Cytosolic sulfotransferases (SULTs) comprise a family of enzymes that catalyze the transfer of a sulfonate group from 3′-phosphoadenosine 5′-phosphosulfate (PAPS) to an acceptor group of the substrate. In doing so, SULTs modulate the activities of a large array of small endogenous and foreign chemicals, including drugs, toxic compounds, steroid hormones, and neurotransmitters. As expected, all SULTs share the same basic fold: a central four-stranded parallel β-sheet surrounded by α-helices and three loops that are often disordered (dashed lines) in the absence of PAP and/or substrate. The crystal structures of SULT1C3 bound to PAP, apo SULT1C2, a ternary complex of SULT1C2 bound to PAP, and the environmental toxin, pentachlorophenol (PCP), and SULT4A1 were solved at 3.2, 2.0, 1.8, and 2.2 Å, respectively.

SULT4A1 is one of the hSULTs that is most divergent in sequence, and examination of the binding pocket revealed two significant differences that are predicted to affect PAP binding. First, a Trp in α3 that is conserved in all other hSULTs and stacks with the adenine ring of PAPS (Trp53 in SULT1A1) is replaced with a Leu in SULT4A1. Second, the magenta PAP binding loop is much shorter in SULT4A1 than in the other hSULTs, and lacks the conserved Lys residue that separates the key PAPS binding residues Arg258 and Gly260 (SULT1A1 numbering), which results in these residues being out of register. Taken together, SULT4A1 has a slightly smaller PAPS binding pocket that is predicted to be unable to accommodate the cofactor. Interestingly, some residual electron density was observed in the PAP binding pocket of recombinant SULT4A1. Presumably this derives from a bound small molecule that was co-crystallized, although we were not able to identify it either by modelling atoms into the electron density or using mass spectrometry. However, PAP when added at concentrations as high as 90 mM did not stabilize SULT4A1. Significantly, this protein, which is expressed primarily in the brain, binds to 2-hydroxylestradiol, thyroid hormone, T4 (3,3′,5,5′-tetraiodo-L-thyronine), and the catecholamines norepinephrine, epinephrine, and isoprenaline (but not dopamine), suggesting that SULT4A1 may modulate the bioactivity of these compounds via a mechanism distinct from sulfonation. SULT4A1 is inactive as an enzyme in our experiments, likely due to its inability to bind PAPS or other sulfonate donors. This orphan SULT likely has an important function in the brain, nevertheless, because it is highly conserved and binds well to the neurotransmitters epinephrine and norepinephrine.

>MAESEAETPSTPGEFESKYFEFHGVRLPPFCRGKMEEIANFPVRPSDVWIVTYPKSGTSLLQEVVYLVSQGADPDEIGLMNIDEQLPVLEYPQPGLDIIKELTSPRLIKSHLPYRFLPSDLHNGDSKVIYMARNPKDLVVSYYQFHRSLRTMSYRGTFQEFCRRFMNDKLGYGSWFEHVQEFWEHRMDSNVLFLKYEDMHRDLVTMVEQLARFLGVSCDKAQLEALTEHCHQLVDQCCNAEALPVGRGRVGLWKDIFTVSMNEKFDLVYKQKMGKCDLTFDFYL[2x]> MELHQIRGCHKNDIELKKYNIGVAISLGNKWFSIDNIEKLVKWSLLHTKEYVIIYIANSIHGINLSV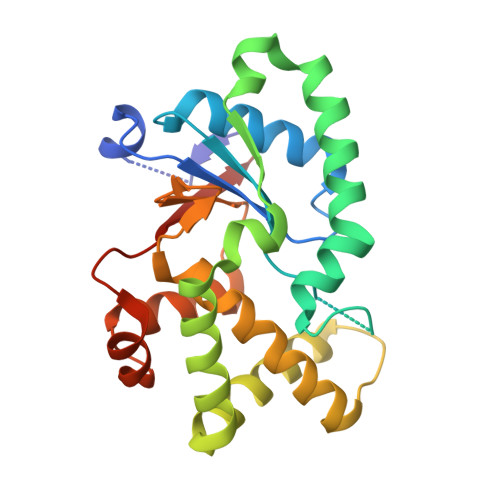RNKLSDSHAEEVAIRYGRNLFIKIKERVSLSFSQDEQAKIIYATWSDIADSKYKEKVKYLYNLYDKNINFKNYIENFVKEWVSKEKRTFNNNEINKFGRYILEELPELMVQVKARGVLFEAYVYPYKTRITEFVGLLQKGEIFPEIKTNILDNHPKIFLEVREHHHHHH>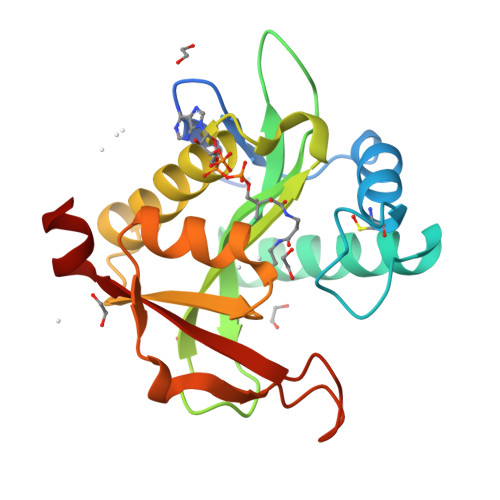[2x]GHMNANLPPSAISELHGPRLLLRAWRDSDREAFAEMCADPQVMEFFPSVLDRAQSDALVDRVQAHFAERGYGPWALELPGEAAFIGFTGLFDVTMDVHFAPTVAIGWRLAPAYWGRGLAREAAETALDFAFERLRLPEVVAFTTPPNRRSWGLMERLGMRRDPAEDFDHPLLAADHPMRRHILYRVDAARWAER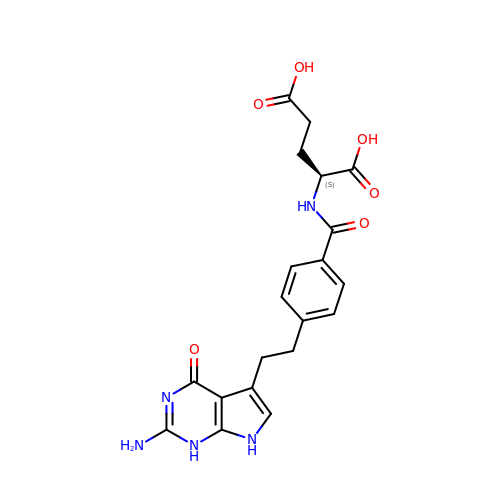2-{4-[2-(2-AMINO-4-OXO-4,7-DIHYDRO-3H-PYRROLO[2,3-D]PYRIMIDIN-5-YL)-ETHYL]-BENZOYLAMINO}-PENTANEDIOIC ACID | C20 H21 N5 O6 | WBXPDJSOTKVWSJ-ZDUSSCGKSA-N>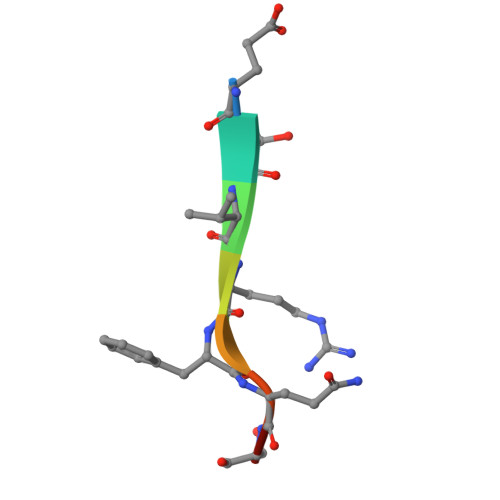 ETVRFQSD>MGSSHHHHHHSSGLVPRGSHHEGHAQAPGTHQTRHGGMTTVGEVDHEKNGFDPYAFLTHWETGEVSTLPSGQTLREFNIVAVDKEIEIAPGVYFPAWTYNGQVPGPTLRVTEGDRVRVHFHNAGSHPHTIHFHGIHPASMDGVPGTGPGMIYPGESFTYEFDAYPFGCHLYHCHAIPLKRHIHKGLYGAFIIDPDPERHPEYQAAARARLLGTPENQAWQEFV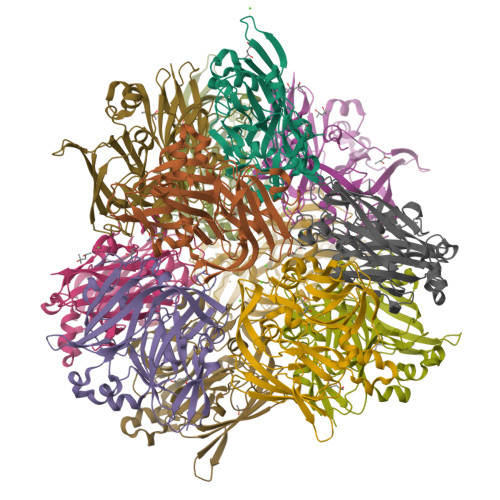MVMNGFDTNFDEENEVYAVNTVAHAYMKRPIRIERDRPVRIYLINATEFDPINSFHLHANFFDYYDHGTTLTPTLKTVDTIMQCQGQRGILEFSFNGFEPGLYMFHAHQSEFAELGWMGNFEVIE[12x]> K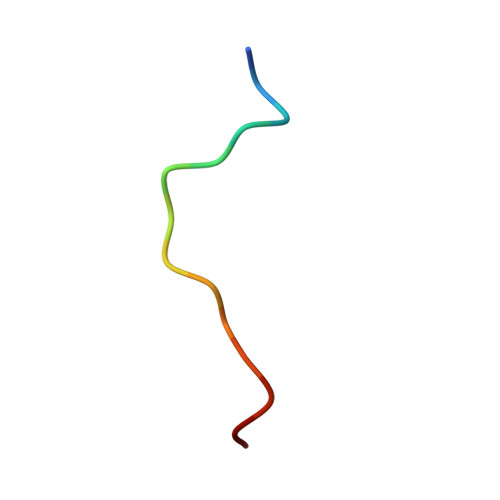AVCSQEAMTGPCR ADP-ribosyl-acceptor hydrolase 3 (ARH3) cleaves PAR and mono(ADP-ribosyl)ation at serine following DNA damage. In contrast, ARH3 has a unique ARH fold and a di-Mg2+-containing catalytic center and can efficiently reverse not only PARylation but also mono(ADP-ribosyl)ation (MARylation) at serine; ARH3 can also cleave O-acetyl-ADPR and α-NAD+ in a Mg2+-dependent manner releasing free ADPR. While coordination of two magnesium ions (MgA and MgB) significantly enhances its catalytic efficiency, calcium binding suppresses its function. In the active site of ARH3, acidic residues, including Asp77, Asp78, Asp314, and Asp316, maintain the integrity of the bimetallic center and render the ideal alignment of the substrate for catalysis.

Similarly, on the other side of the active site, Asp314 interacts with 3″-OH of the terminal ribose and MgB. Asp314 seems to contribute to the integrity of MgB, given that the substitution of Asp314 with glutamate eliminates MgB from the active site. In the structure of ARH3D314A, similar to ARH3D314E, MgB is missing. Unlike ARH3D77A, the orientation of ADPR in ARH3D314A is nearly identical to that in ARH3WT, and critical residues for the formation of the binuclear metal center occupy nearly identical positions. The geometry of MgA is also maintained in an octahedral shape as seen in ARH3WT. The 3″-OH group of the terminal ribose, which is originally in direct coordination with MgB and the side chain of Asp314, lacks interactions with the enzyme in the structure of ARH3D314A and is disordered. Consistent with these findings, ARH3D314A shows a 44-fold decrease in ADPR-binding affinity compared with ARH3WT. Notably, this reduced ADPR-binding affinity mimics the metal-free state of ARH3, further supporting the hypothesis that MgB is critical for substrate binding in ARH3. Among ARH3 mutants, only ARH3D314A showed some residual PAR hydrolysis activity in the presence of Mg2+, and the others were nearly inactive in all three tested metal conditions.

>[4x]GPHMAAAAMAAAAGGGAGAARSLSRFRGCLAGALLGDCVGSFYEAHDTVDLTSVLRHVQSLEPDPGTPGSERTEALYYTDDTAMARALVQSLLAKEAFDEVDMAHRFAQEYKKDPDRGYGAGVVTVFKKLLNPKCRDVFEPARAQFNGKGSYGNGGAMRVAGISLAYSSVQDVQKFARLSAQLTHASSLGYNGAILQALAVHLALQGESSSEHFLKQLLGHMEDLEGDAQSVLDARELGMEERPYSSRLKKIGELLDQASVTREEVVSELGNGIAAFESVPTAIYCFLRCMEPDPEIPSAFNSLQRTLIYSISLGGATDTIATMAGAIAGAYYGMDQVPESWQQSCEGYEETDILAQSLHRVFQKS>LKPEMIEKLNEQMNLELYSSLLYQQMSAWCSYHTFEGAAAFLRRHAQEEMTHMQRLFDYLTDTGNLPRINTVESPFAEY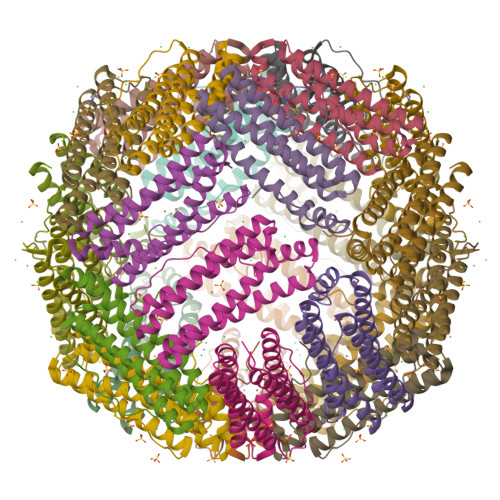SSLDELFQETYKHEQLITQKINELAHAAMTNQDYPTFNFLQWYVSEQHEEEKLFKSIIDKLSLAGKSGEGLYFIDKELSTLDTQN[6x]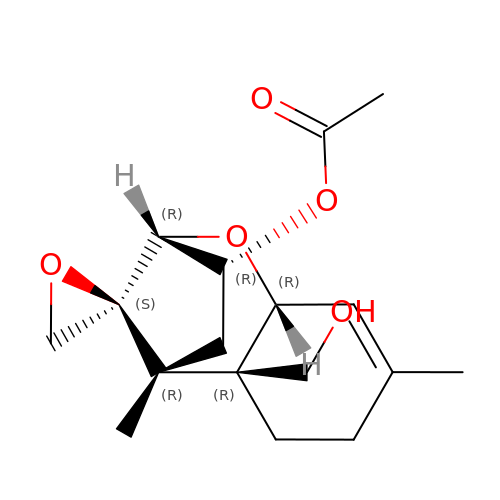(3alpha)-15-hydroxy-12,13-epoxytrichothec-9-en-3-yl acetate | C17 H24 O5 | DFPPNUOWRKIOKO-KWRZAIAESA-N(1~{S})-2,2-bis(fluoranyl)-~{N}-[4-(3-methyl-6-oxidanylidene-2,7-dihydropyrazolo[3,4-b]pyridin-4-yl)cyclohexyl]cyclopropane-1-carboxamide | C17 H20 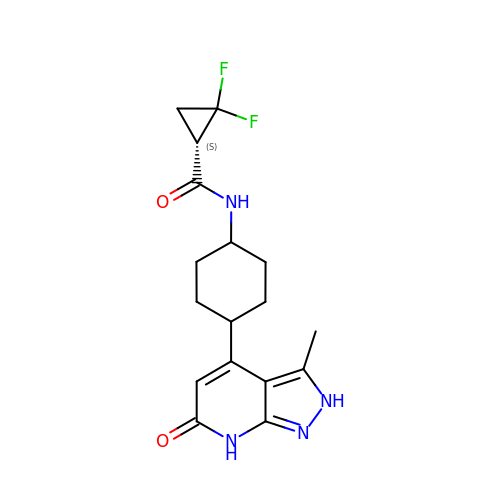F2 N4 O2 | OWAGRTBSGRSEOG-NHCYSSNCSA-N N-[(benzyloxy)carbonyl]-L-aspartic acid 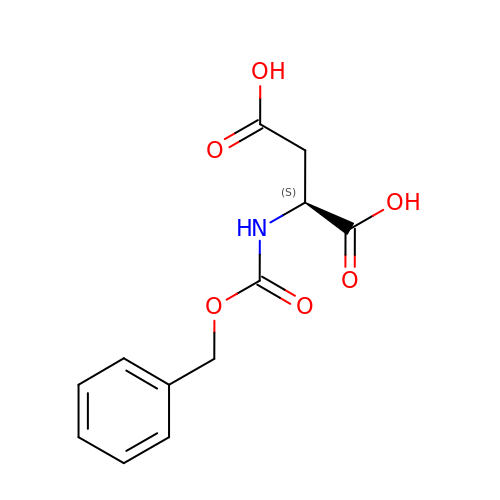| C12 H13 N O6 | XYXYXSKSTZAEJW-VIFPVBQESA-N Sin Nombre virus (SNV) belongs to the Hantaviridae family of the order Bunyavirales, a large and diverse order of segmented negative-strand RNA viruses (sNSVs) containing several emerging pathogens. The multifunctional ~250 kDa L protein of hantaviruses, amongst other functional domains, harbors the RNA-dependent RNA polymerase (RdRp) and an endonuclease and catalyzes transcription as well as replication of the viral RNA genome, making it a promising therapeutic target. The key player in hantavirus replication is the large multifunctional L protein which, together with the nucleoprotein N and viral RNA, forms viral ribonucleoprotein complexes (RNPs). The endonuclease and cap-binding functions are required for viral transcription initiation via cap-snatching to provide short, capped RNA primers derived from host cell mRNAs.

We established an expression and purification protocol, allowing us to obtain highly stable SNV L protein with the endonuclease active site mutation K124A from insect cells. Applying PEGylation, we succeeded to improve grid preparation in lower-salt conditions of the L protein in complex with the 5′ RNA 1–18. Single-particle reconstruction yielded a map at 3.2 Å resolution, comprising parts of the endonuclease linker, the core lobe and vRNA binding lobe (vRBL), the RdRp core with the fingers, palm and thumb domains as well as the bridge, thumb ring and lid domains. No density was visible for the N- and C-terminal regions containing the endonuclease and, presumably, a CBD, respectively. This suggests that these regions are highly flexible in the 5′ RNA-bound conformation of the L protein, as previously reported for other bunyavirus L proteins. The viral 5′ RNA is bound in a pocket formed by the vRBL, core-lobe and fingers domains. Nucleotides 2–12 of the 18mer RNA are visible in the map and form a hook-like conformation stabilized by three base pair interactions between A2 and U12, G3 and C11, and U4 and A10. Protein-RNA contacts between the 5′ hook and SNV L include the side chains of Q388, Y525, and K559 from the vRBL, N290, L403, R567, K617, M618, K619, and K654 from the core lobe, N737 from the fingers domain as well as M1031 and V1038 from the finger node. The fingers domain spans residues 735–920 and 983–1058 and contains the fingertips (residues 884–894) and finger node (1021–48 with missing density for residues 1032 and 1033) insertions that are conserved among sNSVs and the Bunyavirales, respectively. Both insertions were well defined in the map and the loop connecting the two short α-helices of the finger node appears to stabilize the bound 5′ promoter RNA.

> MEKYREIHQRVKEIPPGGASALECLDLLDRLYAVRHDVVDQMIKHDWSDNKDMERPIGQVLLMAGVPNDIIQGMEKKVIPTSPSGQILKSFFRMTPDNYKITGALIEFIEVTVTADVAKGIREAKLKYESGLQFIESLLSQEHKKGNINQVYKITFDVVAVKTDGSNISTQWPSRRNDGVVQHMRLVQADINYVREHLIKPDERASLEAMFNLKFHVGGPKLRYFNIPDYKPQSLCQPEITNLIQYCKHWLTEDHDFVFKEVTGNNVMSSFENNEDVYMSRYKESRKPRNFLLIQGSIQGPYLPSTISSDQCDTRIGCLEVLKVHPETPVQAIAVDMAYKYMELNRDEIINYYNPRVHFQATQSVKEPGTFKLGLSQLNPMSKSILDQVGKHKSEKGLFGEPLESINISSQIQQNECSRIIESILSNLEINVGEVTMNLANPRKTTGVDELLGKFYENELSKYLISILRKTAAWHIGHLIRDITESLIAHAGLKRSKYWSIHAYDHGGVILFILPSKSLEVVGSYIRYFTVFKDGIGLIDEENLDSKVDIDGVQWCFSKVMSIDLNRLLALNIAFEKALLATATWFQYYTEDQGHFPLQHALRSVFSFHFLLCVSQKMKICAIFDNLRYLIPAVTSLYSGYELLIEKFFERPFKSALEVYLYNIIKALLISLAQNNKVRFYSKVRLLGLTVDHSTVGASGVYPSLMSRVVYKHYRSLISEATTCFFLFEKGLHGNLNEEAKIHLETVEWARKFEAKERKYGDILMREGYTIDAIRVGDVQVEQQLFCQEVVELSAEELNKYLQAKSQVLSSNIMNKHWDKPYFSQTRNISLKGMSGALQEDGHLAASVTLIEAIRFLNRSQTNPNVIDMYEQTKQHKAQARIVRKYQRTEADRGFFITTLPTRVRLEIIEDYYDAIARVVPEEYISYGGDKKILNIQTALEKALRWASGSSEITTSTGNVIKFKRRLMYVSADATKWSPGDNSAKFKRFTQALYDGLSDEKLKCCVVDALRHVYETEFFMSRKLHRYIDSMDEHSEAVQDFLDFFKGGVSATVKGNWLQGNLNKCSSLFGAAVSLLFRRIWAELFPELECFFEFAHHSDDALFIYGYLEPEDDGTDWFLYVSQQIQAGNYHWHAVNQEMWKSMFNLHEHLLLMGSIKVSPKKTTVSPTNAEFLSTFFEGCAVSIPFIKILLGSLSDLPGLGFFDDLAAAQSRCVKAMDLGASPQLAQLAVVICTSKVERLYGTADGMVNSPVAFLKVTKAHVPIPLGGDGSMSIMELATAGIGMADKNILKQAFYSYKHTRRDGDRYVLGLFKFLMSLSEDVFQHDRLGEFSFVGKVQWKVFTPKNEFEFYDQFSQSYLKSWTNQHPVYDYIIPRGRDNLLVYLVRKLNDPSIVTAMTMQSPLQLRFRMQAKQHMKVCKLDGEWVTFREVLAAADSFATKYNPTEKDLDLFNTLVSCTFSKEYAWKDFLNEVRCEVVPTKHVHRSKIARTFTVREKDQAIQNPITAVIGYKYASTVDEISDVLDSSFFPDSLSADLQVMKEGVYRELGLDIGLPEVLKRIAPLLYKAGRSRVVIVEGNVEGTAESICSYWLRSMSLVKTIKVRPKKEVLRAVSLYSTKENIGLQDDVAATRLCIEVWRWCKANDQNVNDWLNALYFEKQTLMDWVERFRRKGVVPVDPEIQCIALLLYDVLGYKSVLQMQANRRAYSGKQYDAYCVQTYNEETKLYEGDLRVTFNFGLDCARLEIFWDKKEYILETSITQRHVLKLMMEEVTQELLRCGMRFKTEQVSHTKSLVLFKTESGFEWGKPNVPCIVFKHCALRTGLRTKQAINKEFMINVQADGFRAIAQMDVESPRFLLAHAYHTLRDVRYQAVQAVGNVWFQTNQHKLFINPIISSGLLENFMKGLPAAIPPAAYSLIMNKAKISVDLFMFNELLALVNPRNVLNLDGIEETSEGYSTVTSISSRQWSEEVSLMADDNIDDEEEFTIALDDIDFEQINLDEDIQHFLQDESAYTGDLTIQTEEVEVKRIRGVTRVLEPVKLIKSWVSKGLAIDKVYNPIGIVLMARYMSKNYDFSKIPLALLNPYDLTEFESVVKGWGETVNDRFLEVDNDAQRLIREKNILPEDILPDSLFSFRHVDVLLKRLFPRDPVSSFY> SNAMFAPQGLAQFIKVNVTLENGEPVFIYTDANGQ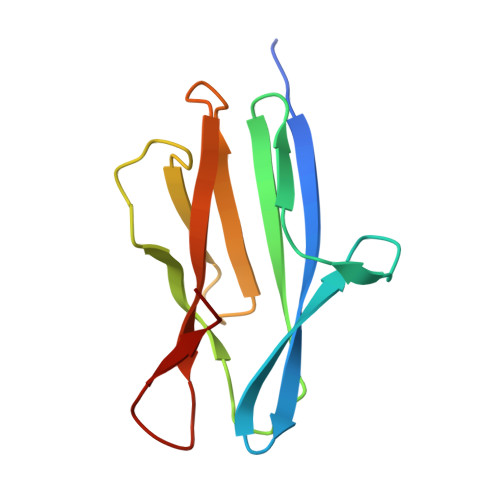VCQGDITVTQAGTITYLLNDQTLKGLKFVGVGFVTPFDGIIDAVTISSDGMLVQLVDLDKTPGTTKFQFVLSNTANTLLVLSPD>[3x]MDKGKSV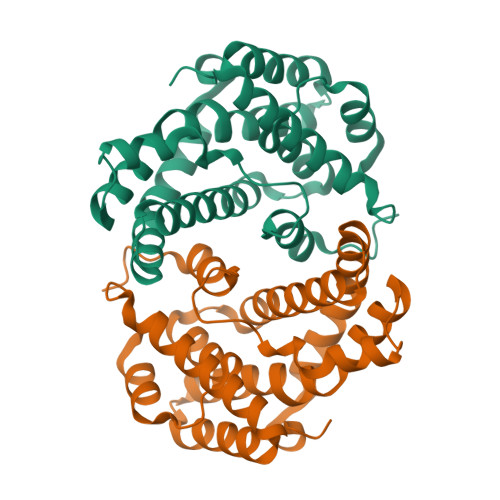KSTEKSVGMPPKTPKTDNNAHVDNEFLILQVNDAVFPIGSYTHSFGLETYIQQKKVTNKESALEYLKANLSSQFLYTEMLSLKLTYESALQQDLKKILGVEEVIMLSTSPMELRLANQKLGNRFIKTLQAMNELDMGEFFNAYAQKTKDPTHATSYGVFAASLGIELKKALRHYLYAQTSNMVINCVKSVPLSQNDGQKILLSLQSPFNQLIEKTLELDESHLCTASVQNDIKAMQHESLYSRLYMS>GPLGSMTIIESNYISVREEYPDIDSEVRAILLSHAQNGITISSIKSEYRKLTGNPFPLHDNVTDFLLTIPNVTAECSESGKRIFNLKASLKNGHLLDMVLNQKERTS[2x];>[2x]GHSDVKQTIYEVNKYAKRSKLIEILSEQADGTIVFVETKRGADFLASFLSEKEFPTTSIHGDRLQSQREQALRDFKNGSMKVLIATSVASRGLDIKNIKHVINYDMPS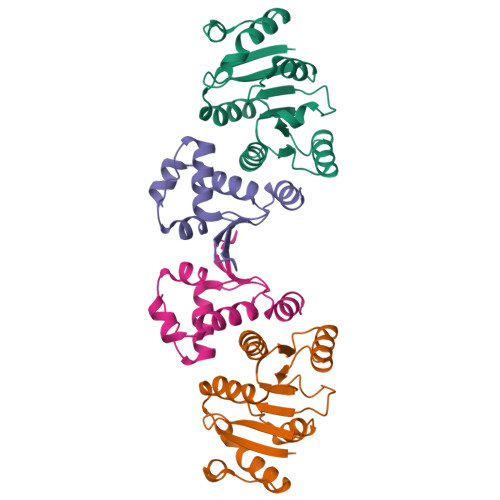KIDDYVHRIGRTGRVGNNGRATSFFDPEKDRAIAADLVKILEGSGQTVPDFLRTC>[4x]MNHKVHHHHHHIEGRHMASAGDVTRAALPRAQPRAEGPACVLGIGTAVPPAEFLQSEYPDFFFNITNCGEKEALKAKFKRICDKSGIRKRHMFLTEEVLKANPGICTYMEPSLNVRHDIVVVQVPKLAAEAAQKAIKEWGGRKSDITHIVFATTSGVNMPGADHALAKLLGLKPTVKRVMMYQTGCFGGASVLRVAKDLAENNKGARVLAVASEVTAVTYRAPSENHLDGLVGSALFGDGAGVYVVGSDPKPEVEKPLFEVHWAGETILPESDGAIDGHLTEAGLIFHLMKDVPGLISKNIEKFLNEARKPVGSPAWNEMFWAVHPGGPAILDQVEAKLKLTKDKMQGSRDILSEFGNMSSASVLFVLDQIRHRSVKMGASTLGEGSEFGFFIGFGPGLTLEVLVLRAAPNSA;>[4x]MNHKVHHHHHHIEGRHMGLQVVNVEGIDFATKFAPPTSSTELDLIGHGNTGMEIETVE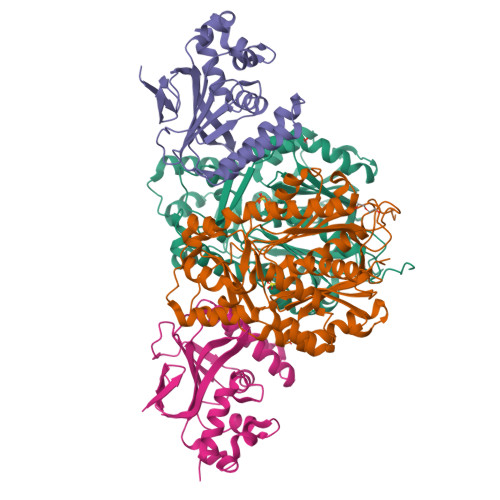IRFTAMGFYAEPSISEHLQKWKGKAVSELVEDDSGFHKELIQVPVEKAVRISIIKGIKGLPYGSALQSSLRDRLVNDDKFEEEEEEALEKLVEFFQPHNLPKGANIIYHWATPDTVKISLSEEGKIPDEVSYTIEDANVAEALLDLYLGENTITPSTLSSVAEAIAAQVA>GPHMGDKLFQLFQLCLSAISQCSGTPELRSLYYSICYRYLTAVVDNDATVAATPASSTIGPTRSVTNARARTLKAITLYGDRLLNVICDDAYGSDTTCQTAAMILLNALVHTSRASSAAGVSPADVDCPIIDALNRLNFIGVLVDSLKEILNEWLAPSSTFDPSLSTNASPSLPIPASPSQQYTSAKLALLLQLCQTRQGAKYVLQANLFRALEQSGVFAADPELVEVDSESGVPRVVALERHYALLVALARVVGAAVTARGAHNIVQGRKFLTQHRGLVVHVLKKNAGIGGGVVGNSLASSING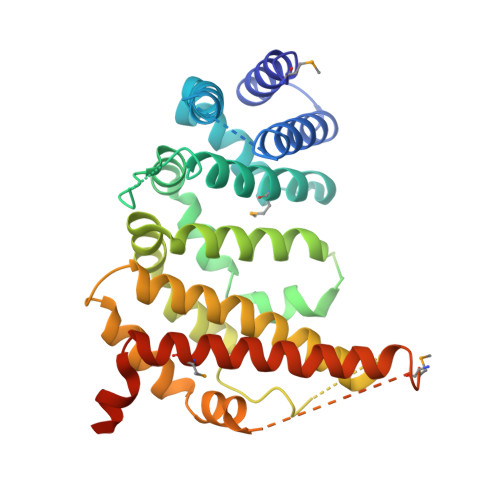GSTATMTRRDEILAQQALEERIEELAEAFMLLITATGFLEYESEQVPSEQPRAHTTFFH[2x]SKD3, also known as CLPB, is a ring-forming, ATP-fueled protein disaggregase essential for preserving mitochondrial integrity and structure. Ankyrin repeats are one of the most abundant motifs found in eukaryotic proteins and the Ank domain is the defining feature that distinguishes mammalian SKD3 from microbial Hsp100 unfoldases. Here, we present the atomic structures of the isolated Ank domains of SKD3 isoform-1 (ANKiso1) and SKD3 isoform-2 (ANKiso2). The two isoforms differ by a 30 amino acid stretch present in isoform-1 (exon-5), which represses the protein disaggregating activity of SKD3.

Owing to a lack in our molecular understanding of the Ank domain, we solved the crystal structure of ANKiso1 at 1.81-Å resolution using the single wavelength anomalous diffraction (SAD) technique. Although the crystal structure contains only one ANKiso1 molecule in the crystallographic asymmetric unit, it appears to form a dimer in solution. Amongst the Ank motifs, Ank2 is most unusual and features a long β-hairpin-helix motif instead of the canonical loop. The electron density for helix α5 (residues 232-240) is clearly visible in our experimentally phased map, which is sandwiched between the β-hairpin and the concave surface of the Ank domain. The interaction is mediated by hydrophobic contacts between the side chains of Phe236, Arg237 and Trp239 of α5 and His300 as well as Tyr305 from η1. In the crystal, this sandwich conformation is stabilized by the C-terminal segment of a symmetry-related neighboring Ank domain, which wraps around the β-hairpin, and may provide a structural basis for dimer formation in solution. Although the overall structure of ANKiso1 resembles the AlphaFold2 model (AF-Q9H078-F1), we note that the long β-hairpin with the intervening α5 helix is unexpected and markedly differs in both the location and secondary structure from the predicted AlphaFold2 model. The structure of ANKiso1 suggested that binding of helix α5 may compete with substrate interaction. The crystal structures of the Ank domain showed that all three MGCA7-associated missense mutations map to the Ank2 motif and cluster around Cys267 that follows the long β-hairpin. Interestingly, the Cα distance between Cys267 and Tyr272 is 7.0-Å, which is within the range of Cα distances between disulfide bonded cysteines observed in protein structures.

> AAASNKDAALLEAARANNMQEVSRLLSEGADVNAKHRLGWTALMVAAINRNNSVVQVLLAAGADPNLGDDFSSVYKTAKEQGIHSLEDGGQDGASRHITNQWTSALEFRRWLGLPAGVLITREDDFNNRLNNRASFKGCTALHYAVLADDYRTVKELLDGGANPLQRNEMGHTPLDYAREGEVMKLLRTSEAKYQEKQRKREAEERRRFPLEQRLKEHIIGQE> AFVVTDNCIKCKYTDCVE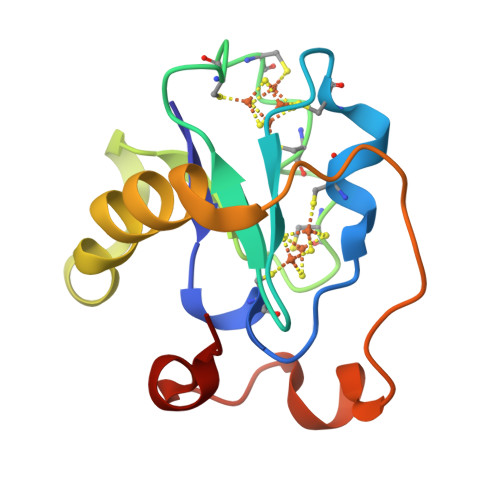VCPVDCFYEGPNFLVIDPDECIDCALCEPECPAQAIFSEDEVPEDMQEFIQLNAELAEVWPNITEKKDPLPDAEDWDGVKGKLQHLER>[2x]EKNVKEITDATKEPYNSVVAFVGGTGVVVGKNTIVTNKHIAKSNDIFKNRVSAHHSSKGKGGGNYDVKDIVEYPGKEDLAIVHVHETSTEGLNFNKNVSYTKFADGAKVKDR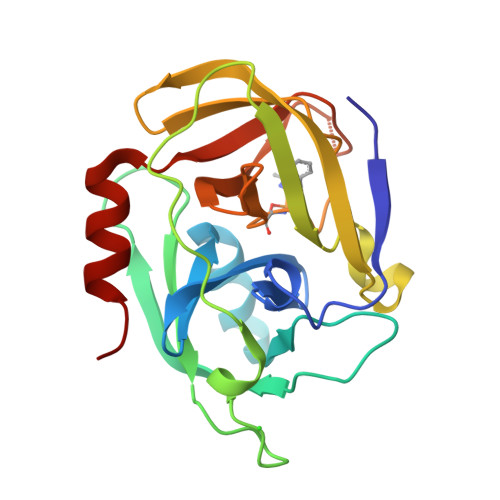ISVIGYPKGAQTKYKMFESTGTINHISGTFMEFDAYAQPGNSGSPVLNSKHELIGILYAGSGKDESEKNFGVYFTPQLKEFIQNNIEK>GMSHKILELYSGIGGMHCAWKESGLDGEIVAAVDINTVANSVYKHNFPETNLLNRNIQQLTPQVIKKW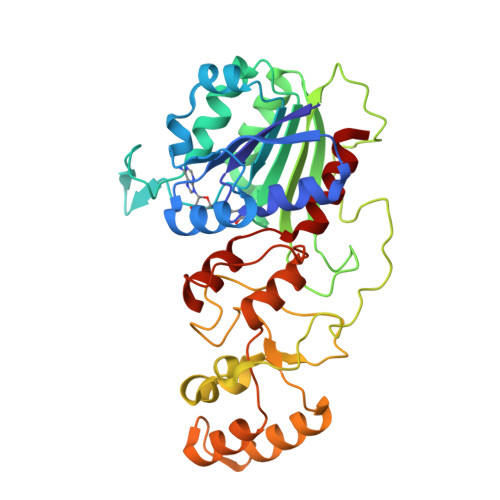NVDTILMSPPCQPFTRNGKYLDDNDPRTNSFLYLIGILDQLDNVDYILMENVKGFENSTVRNLFIDKLKECNFIYQEFLLCPSTVGVPNSRLRYYCTARRNNLTWPFKRRDEIITRLPKDFGVPHSLESIIEEDVDEKFLVPEKMLRCAKVFDICYKTSKRSCCFTKAYTHYADGTGSIFTDKPREVVQKCYAAAAQNEIGGEKFVELFKELKLRYFTPKEVLMIMCFPKSYNLPTNISMKQCYRLLGNSVNVKVISELLKILFE[4x]> ILQTTVDGNSTAISNLKSDISSNGLAITDLQDRVKSLESTASHGLSFSPPLSVADGVVSLDMDPYFCSQRVSLTSYSAEAQLMQFRWMARGTNGSSDTIDMTVNAHCHGRRTDYMMSSTGNLTVTSNVVLLTFDLSDITHIPSDLARLVPSAGFQAASFPVDVSFTRDSATHAYQAYGV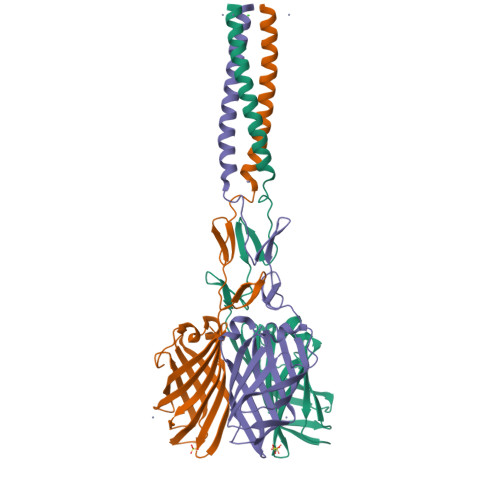YSSSRVFTITFPTGGDGTANIRSLTVRTGIDT> GSNSHSYLSGYISLLLRAEPYPTSRFGSQCMQPNNIMGIENICELAARMLFSAVEWARNIPFFPDLQITDQVALLRLTWSELFVLNAAQCSMPLHVAPLLAAAGLHASPMSADRVVAFMDHIRIFQEQ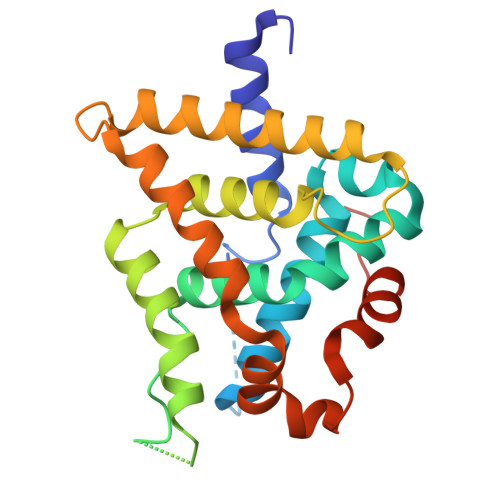VEKLKALHVDSAEYSCLKAIVLFTSDACGLSDVAHVESLQEKSQCALEEYVRSQYPNQPTRFGKLLLRLPSLRTVSSSVIEQLFFVRLVGKTPIETLIRDMLLSGSSFNWPYMAIQ>MSQSGEDLHSPTYLSWRKLQLSRAKLKASSKTSALLSGFAMVAMVEVQLDHDTNVPPGMLIAFAICTTLLVAVAMLALMISTCILPNIETVSNLHSISLVHESPHERLHWYIETAWAFSTLLGLILFLLEIAILCWVKFYDLSPPAAWSATVVLIPVMII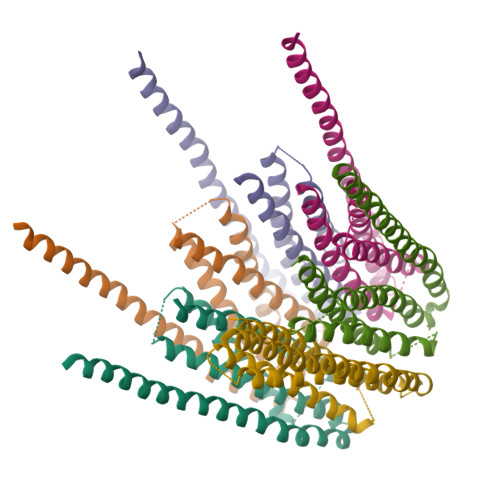FMAFAIHFYRSLVSHKYEVTVSGIRELEMLKEQMEQDHLEHHNNIRNNGEGEEF[24x]> GKRPRPVMCQCVDTTNGGVRLDAVTRAACSIDSFIDGYYTEKDGFCRAKYSWDLFTSGQF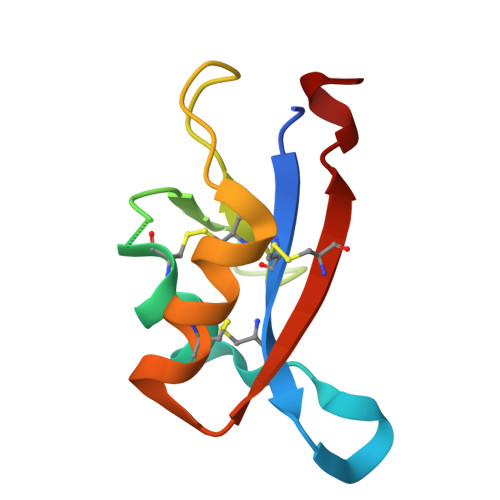YQACLRYSHAGTNCQPDPQYE4-({[4-(4-chlorophenoxy)phenyl]sulfanyl}methyl)-N-hydroxytetrahydro-2H-pyran-4-carboxamide | C19 H20 Cl N O4 S | 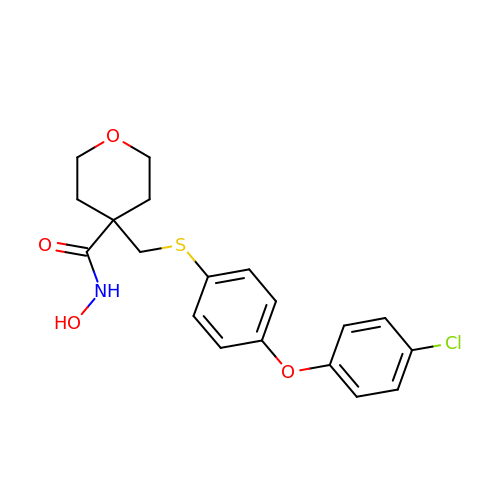PMNRYCFAWDUYAJ-UHFFFAOYSA-N> MSEFSQTVPELVAWARKNDFSISLPVDRLSFLLAVATLNGERLDGEMSEGELVDAFRHVSDAFEQTSETIGVRANNAINDMVRQRLLNRFTSEQAEGNAIYRLTPL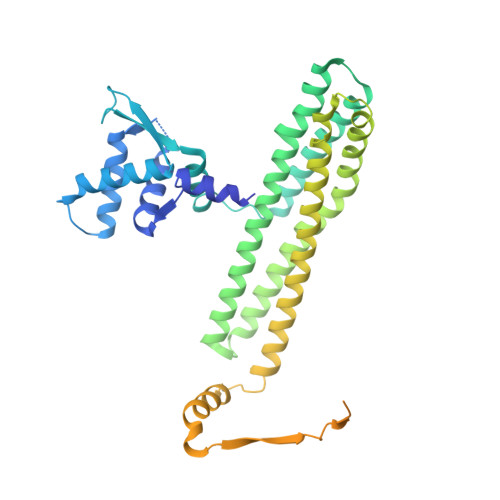GIGITDYYIRQREFSTLRLSMQLSIVAGELKRAADAAEEGGDEFHWHRNVYAPLKYSVAEIFDSIDLTQRLMDEQQQQVKDDIAQLLNKDWRAAISSCELLLSETSGTLRELQDTLEAAGDKLQANLLRIQDATMTHDDLHFVDRLVFDLQSKLDRIISWGQQSIDLWIGYDRHVHKFIRTAIDMDKNRVFAQRLRQSVQTYFDEPWALTYANADRLLDMRDEEMALRDEEVTGELPEDLEYEEFNEIREQLAAIIEEQLAVYKTRQVPLDLGLVVREYLSQYPRARHFDVARIVIDQAVRLGVAQADFTGLPAKWQPINDYGAKVQAHVIDKY>MKKYGFNFQWMYVWEEGREPEPPDKKALDFLAETGFNFVRIPVDYRFWTRNFDYFNPDKKVFEYIDLYLRECSARNIHMCLNLHRAPGYCINRNDIERDNLWLDKRAQDG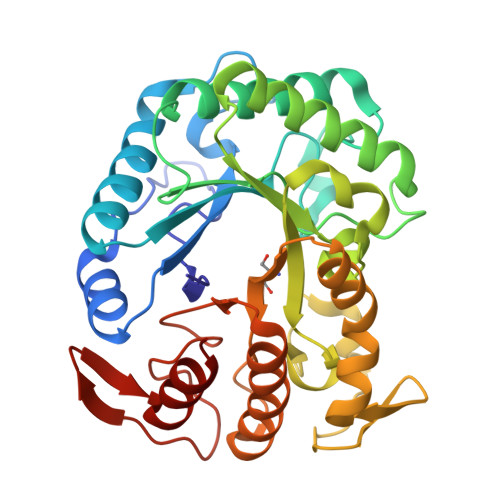FVYQWELFAKRYKGVSSKFLSFDLVNEPPNIGQYGLTRENHASLIIRTVEAIRKIDPDREIVIDGLGGGNIAMPELAHLGVVHSGRGYQPMALTHYQASWWDGHKGLPEPYYPDLLWQGKVWNKDTLREYYKPWRDLQQKGVNVHIGEFGCFNKTSNDVAIRWFEDVLSLYKEFEWGYSLWNFKGPFGIVEHGRPGAKYEYYRGFKVDRELLDLLVENRV[2x]>[2x]VVKRTMTKKFLEEAFAGESMAHMRYLIFAEKAEQEGFPNIAKLFRAIAYAEFV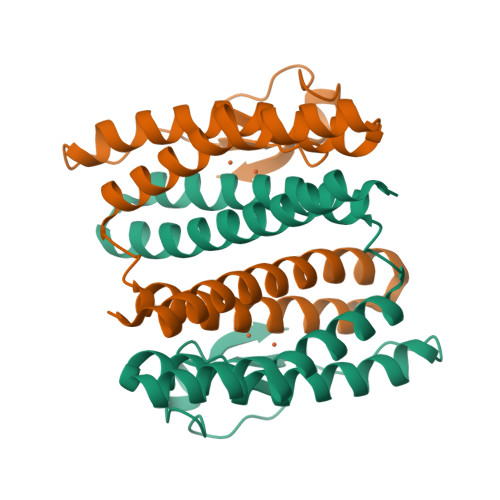HAKNHFIALGKLGKTPENLQMGIEGETFEVEEMYPVYNKAAEFQGEKEAVRTTHYALEAEKIHAELYRKAKEKAEKGEDIEIKKVYICPICGYTAVDEAPEYCPVCGAPKEKFVVFE> GGCCGUGCUAAGCGGGGAGGUAGCGGUGCCCUGUACCUGCAAUCCGCUCUAGCAGGGCCGAAUCCCUUCUCGAGGUUCGGUAACG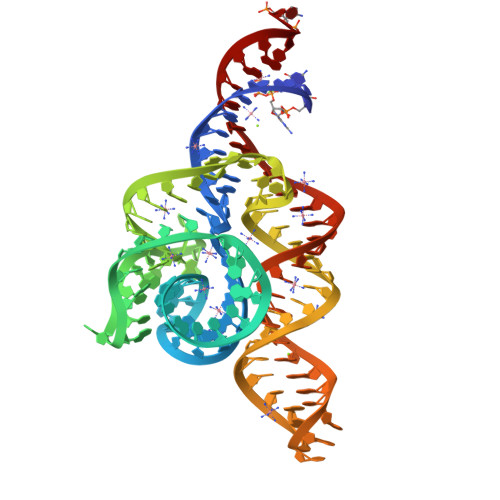AAUCGACAGAAGGUGCACGGUC>[4x]MEKDTKQVDIIFRSKLPDIYIPNHLPL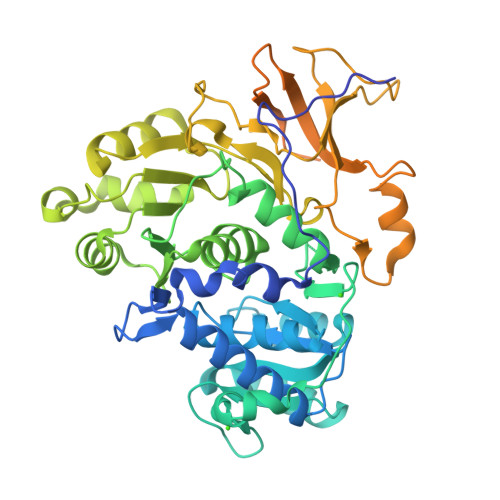HSYCFENISEFSSRPCLINGANKQIYTYADVELNSRKVAAGLHKQGIQPKDTIMILLPNSPEFVFAFIGASYLGAISTMANPLFTPAEVVKQAKASSAKIIVTQACHVNKVKDYAFENDVKIICIDSAPEGCLHFSVLTQANEHDIPEVEIQPDDVVALPYSSGTTGLPKGVMLTHKGLVTSVAQQVDGENPNLYIHSEDVMLCVLPLFHIYSLNSVLLCGLRVGAAILIMQKFDIVSFLELIQSYKVTIGPFVPPIVLAIAKSPMVDDYDLSSVRTVMSGAAPLGKELEDTVRAKFPNAKLGQGYGMTEAGPVLAMCLAFAKEPFEIKSGACGTVVRNAEMKIVDPKTGNSLPRNQSGEICIRGDQIMKGYLNDPEATARTIDKEGWLYTGDIGYIDDDDELFIVDRLKELIKYKGFQVAPAELEALLLNHPNISDAAVVPMKDEQAGEVPVAFVVRSNGSTITEDEVKDFISKQVIFYKRIKRVFFVDAIPKSPSGKILRKDLRAKLAAGLPN>[2x]MGDKPIWEQIGSSFIQHYYQLFANDRTQLGAIYIDASCLTWEGQQFQGKAA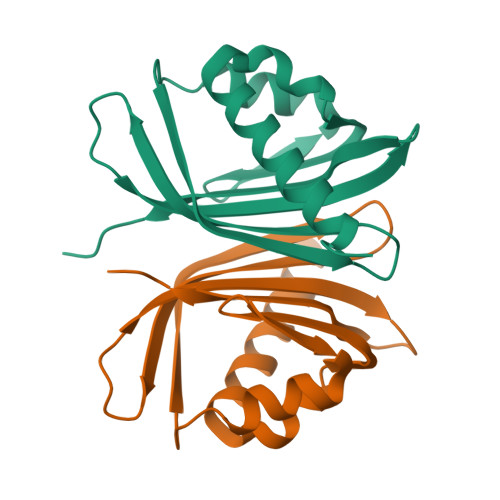IVEKLSSLPFQKIQHSITAQDHQPTPDSCIISMVVGQLKADEDPIMGFHQMFLLKNINDAWVCTNDMFRLALHNFG> NARKVQMGAKDATPVPCGRWAKILEKDKRTQQMRMQRLKAKLQMPFQSGEFKALTRRLQVEPRLLSKQMAGCLEDCTRQAPESPWEEQLARLLQEAPGKLSLDVEQAPSGQHSQAQLSGQQQRLLAFFKCCLLTDQLPLAHHLLVVHHGQRQKRKLLTLDMYNAVMLGWARQGAFKELVYVLFMVKDAGLTPDLLSYAAALQCMGRQDQDAGTIERCLEQMSQEGLKLQALFTAVLLSEEDRATVLKAVHKVKPTFSLPPQLPPPVNTSKLLRDVYAKDGRVSYPKLHLPLKTLQCLFEKQLHMELASRVCVVSVEKPTLPSKEVKHARKTLKTLRDQWEKALCRALRETKNRLEREVYEGRFSLYPFLCLLDEREVVRMLLQVLQALPAQGESFTTLARELSARTFSRHVVQRQRVSGQVQALQNHYRKYLCLLASDAEVPEPCLPRQYWEALGAPEALREQPWPLPVQMELGKLLAEMLVQATQMPCSLDKPHRSSRLVPVLYHVYSFRNVQQIGILKPHPAYVQLLEKAAEPTLTFEAVDVPMLCPPLPWTSPHSGAFLLSPTKLMRTVEGATQHQELLETCPPTALHGALDALTQLGNCAWRVNGRVLDLVLQLFQAKGCPQLGVPAPPSEAPQPPEAHLPHSAAPARKAELRRELAHCQKVAREMHSLRAEALYRLSLAQHLRDRVFWLPHNMDFRGRTYPCPPHFNHLGSDVARALLEFAQGRPLGPHGLDWLKIHLVNLTGLKKREPLRKRLAFAEEVMDDILDSADQPLTGRKWWMGAEEPWQTLACCMEVANAVRASDPAAYVSHLPVHQDGSCNGLQHYAALGRDSVGAASVNLEPSDVPQDVYSGVAAQVEVFRRQDAQRGMRVAQVLEGFITRKVVKQTVMTVVYGVTRYGGRLQIEKRLRELSDFPQE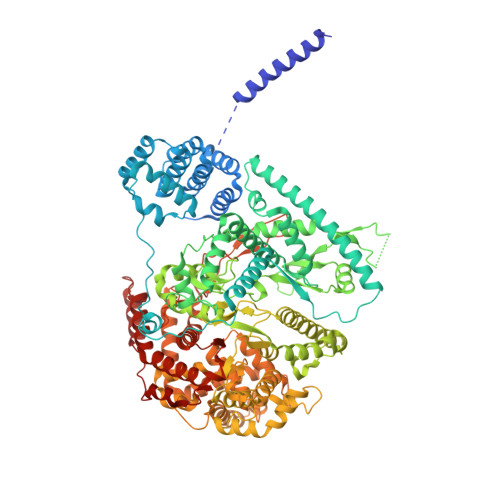FVWEASHYLVRQVFKSLQEMFSGTRAIQHWLTESARLISHMGSVVEWVTPLGVPVIQPYRLDSKVKQIGGGIQSITYTHNGDISRKPNTRKQKNGFPPNFIHSLDSSHMMLTALHCYRKGLTFVSVHDCYWTHAADVSVMNQVCREQFVRLHSEPILQDLSRFLVKRFCSEPQKILEASQLKETLQAVPKPGAFDLEQVKRSTYFFS>[2x]MPHFTVTKVEDPEEGAAASISQEPSLADIKARIQDSDEPDLSQNDITGEHSQLLDDGHKKARNAYLNNSNYEEGDEYFDKNLALFEEEMDTRPKVSSLLNRMANYTNLTQGAKEHEEAENITEGKKKPTKTPQMGTFMGVYLPCLQNIFGVILFLRLTWVVGTAGVLQAFAIVLICCCCTMLTAISMSAIATNGVVPAGGSYFMISRALGPEFGGAVGLCFYLGTTFAAAMYILGAIEIFLVYIVPRAAIFHSDDALKESAAMLNNMRVYGTAFLVLMVLVVFIGVRYVNKFASLFLACVIVSILAIYAGAIKSSFAPPHFPVCMLGNRTLSSRHIDVCSKTKEINNMTVPSKLWGFFCNSSQFFNATCDEYFVHNNVTSIQGIPGLASGIITENLWSNYLPKGEIIEKPSAKSSDVLGSLNHEYVLVDITTSFTLLVGIFFPSVTGIMAGSNRSGDLKDAQKSIPIGTILAILTTSFVYLSNVVLFGACIEGVVLRDKFGDAVKGNLVVGTLSWPSPWVIVIGSFFSTCGAGLQSLTGAPRLLQAIAKDNIIPFLRVFGHSKANGEPTWALLLTAAIAELGILIASLDLVAPILSMFFLMCYLFVNLACALQTLLRTPNWRPRFRYYHWALSFMGMSICLALMFISSWYYAIVAMVIAGMIYKYIEYQGAEKEWGDGIRGLSLSAARFALLRLEEGPPHTKNWRPQLLVLLKLDEDLHVKHPRLLTFASQLKAGKGLTIVGSVIVGNFLENYGEALAAEQTIKHLMEAEKVKGFCQLVVAAKLREGISHLIQSCGLGGMKHNTVVMGWPNGWRQSEDARAWKTFIGTVRVTTAAHLALLVAKNISFFPSNVEQFSEGNIDVWWIVHDGGMLMLLPFLLKQHKVWRKCSIRIFTVAQLEDNSIQMKKDLATFLYHLRIEAEVEVVEMHDSDISAYTYERDLMMEQRSQMLRHMRLSKTERDREAQLVKDRNSMLRLTSIGSDEDEETETYQEKVHMDWTKDKYMASRGQKAKSMEGFQDLLNMRPDQSNVRRMHTAVKLNEVIVNKSHEAKLVLLNMPGPPRNPEGDENYMEFLEVLTEGLERVLLVRGGGSEVITIYS

Potassium‐coupled chloride transporters (KCCs) play crucial roles in regulating cell volume and intracellular chloride concentration. They are characteristically inhibited under isotonic conditions via phospho‐regulatory sites located within the cytoplasmic termini. Decreased inhibitory phosphorylation in response to hypotonic cell swelling stimulates transport activity, and dysfunction of this regulatory process has been associated with various human diseases. Here, we present cryo‐EM structures of human KCC3b and KCC1, revealing structural determinants for phospho‐regulation in both N‐ and C‐termini.

To understand the structural basis of phospho‐regulation in potassium‐coupled chloride transporters, we used single‐particle cryo‐electron microscopy to study the full‐length wild‐type KCC3b transporter and mutants of this transporter in which two canonical threonines (T940 and T997) and a third KCC3‐specific phosphorylation site (S45), which was shown to play a role for full activation in response to swelling (Melo et␣al, 2013), were replaced. Unfortunately, the bias towards top views was even worse for mutant KCC3b‐PKO and prevented 3D reconstruction beyond 6.5 Å. However, we achieved a map resolution of 3.2 Å for the phospho‐inhibited KCC3b‐PM variant (Fig 1B and Appendix␣Fig S4). A unique feature observed in the phospho‐mimetic KCC3b‐PM structure is the presence of pronounced density for a short stretch of the otherwise unstructured N‐terminus, a domain that has not been resolved in any of the previously published CCC structures. Distinct helical‐shaped electron densities are visible near the intracellular cavity created by the hinged helices TM1a and TM6b in both chains of the KCC3 dimer (red surfaces in Figs 1B and 2A), which allowed us to build approximately 30 amino acids of the N‐terminus, assisted by the Rosetta FastRelax protocol (Conway et␣al, 2014) (Appendix␣Fig S5). Electrostatic surface representations of KCC3b in absence or presence of the N‐terminus illustrate that this segment is wedged between CTD and TMD and partially inserted into the inward‐open vestibule created by the helical arrangement of TM2, TM7 and the helices TM1a and TM6b of the transporter core domain. The direct contact with the ion coordinating helices TM1a and TM6b results in a visible obstruction of the ion access path from the intracellular side, suggesting that this domain arrangement could play a role in controlling transport activity. In line with an obstructed ion path, the KCC3b‐PM map does not show any densities for cations coordinated by highly conserved residues of the cation‐binding site: Y232, I148, P443 and T446 (Fig EV2E). By contrast, no densities for ATP or ADP are visible in the map of KCC3b‐PM, which could be the result of small sequence differences in KCC3b.>GPGMSSLSNSLPLMEDVQGIRKAQKADGTATVMAIGTAHPPHIFPQDTYADVYFRATNSEHKVELKKKFDHICKKTMIGKRYFNYDEEFLKKYPNITSYDEPSLNDRQDICVPGVPALGTEA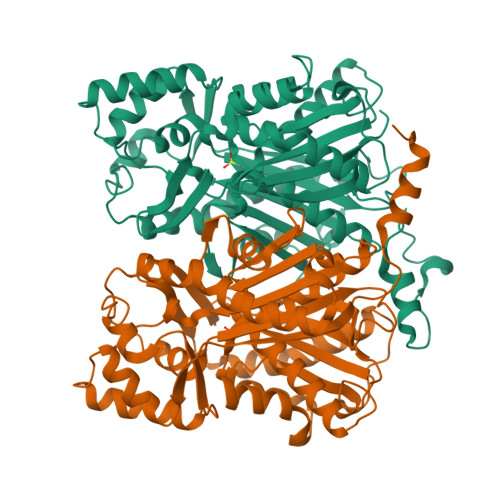AVKAIEEWGRPKSEITHLVFCTSCGVDMPSADFQCAKLLGLHANVNKYCIYMQGCYAGGTVMRYAKDLAENNRGARVLVVCAELTIMGLRAPNETHLDNAIGISLFGDGAAALIIGSDPIIGVEKPMFEIVCTKQTVIPNTEDVIHLHLRETGMMFYLSKGSPMTISNNVEACLIDVFKSVGITPPEDWNSLFWIPHPGGRAILDQVEAKLKLRPEKFRAARTVLWDYGNMVSASVGYILDEMRRKSAAKGLETYGEGLEWGVLLGFGPGITVETILLHSLPLM[2x]(2S,3R,4R)-2,3,4,5-tetrahydroxy-N-oxo-pentanamide 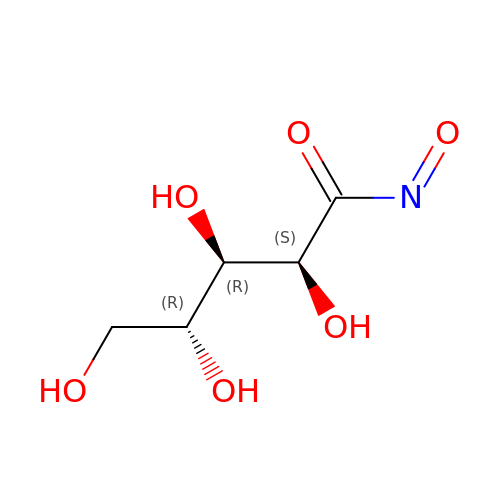| C5 H9 N O6 | VIMQVNVKLDVNFU-JJYYJPOSSA-N>EGDIHMELLKKRATRKAREITSDMEEDKDLMLKLLDKNGFVLKKVEIYRSNYLAILEKRTNGIRNFEINNNGNMRIFGYKMMEHHIQKFTDIGMSCKIAKNGNVYLDI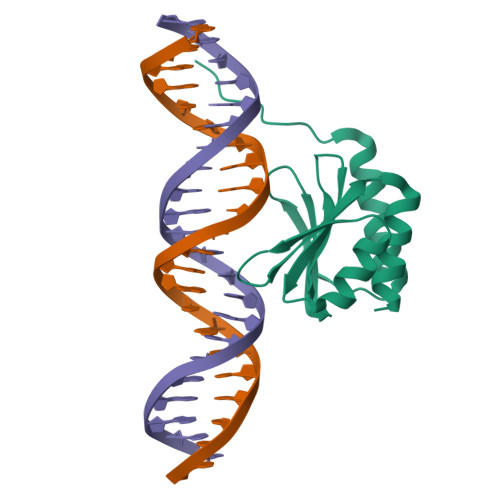KRSAENIEAVITVASEL[4x]>MTVRTRVTDLLEIEHPILMGGMAWAGTPTLAAAVSEAGGLGIIGSGAMKPDDLRKAISELRQKTDKPFGVNIILVSPWADDLVKVCIEEKVPVVTFGAGNPTKYIRELKENGTKVIPVVASDSLARMVERAGADAVIAEGMESGGHIGEVTTFVLVNKVSRSVNIPVIAAGGIADGRGMAAAFALGA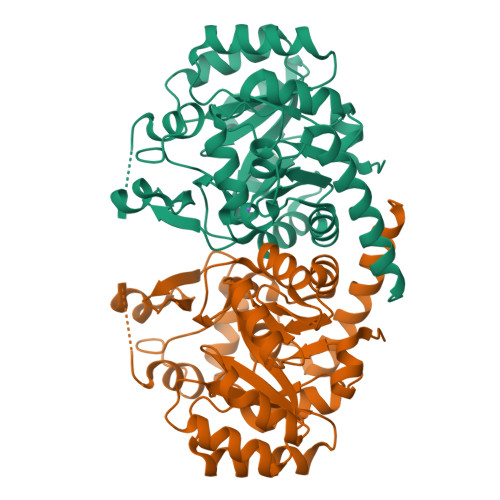EAVQMGTRFVASVESDVHPVYKEKIVKASIRDTVVTGAKLGHPARVLRTPFARKIQEMEFENPMQAEEMLVGSLRRAVVEGDLERGSFAVGQSAGLIDEIKPVKQIIEDILKEFKETVEKLRGYIEE[2x]>[6x]MPRVLVTGALGQIGTDLSLALRDKFGADSVLVSDVVEPGAKHPLAGLKGVEKLDCLDSNGFEKLVKEFKPTWMYHLPAIMSVRGEAEPDLAMDINVNTTRYALELARKYNIRIFIPSTIAAFGDKC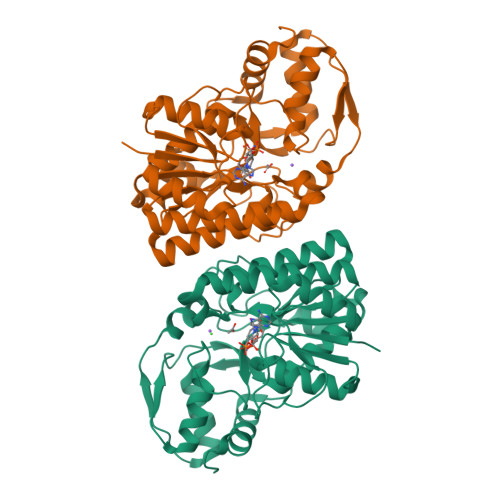GKTMTKDDTIMNPSTVYGVTKVYTELLGTWYRQKYGVDFRSVRLPGIISAATLPGGGATDYAIHMYHSALLQKKCVCPVLPYESLPMMYMPDTLNSLVKIMEAPLEKLTRTVYNITGFSFSPSELRFSIERCTDRTIEVEYVEGPAQKIANSWPDSLDDSNARNDWGHQVKYDIDMMSEDMLRQIPILHGLPSL> HHAADYVLYKDATKPVEDRVADLLGRMTLAEKIGQMTQIERLVATPDVLRDNFIGSLLSGGGSVPRKGATAKEWQDMVDGFQKACMSTRLGIPMIYGIDAVHGQNNVYGATIFPHNVGLGATRDPYLVKRIGEATALEVRATGIQYAFAPCIAVCRDPRWGRCYESYSEDRRIVQSMTELIPGLQGDVPKDFTSGMPFVAGKNKVAACAKHFVGDGGTVDGINENNTIINREGLMNIHMPAYKNAMDKGVSTVMISYSSWNGVKMHANQDLVTGYLKDTLKFKGFVISDWEGIDRITTPAGSDYSYSVKASILAGLDMIMVPNKYQQFISILTGHVNGGVIPMSRIDDAVTRILRVKFTMGLFENPYADPAMAEQLGKQEHRDLAREAARKSLVLLKNGKTSTDAPLLPLPKKAPKILV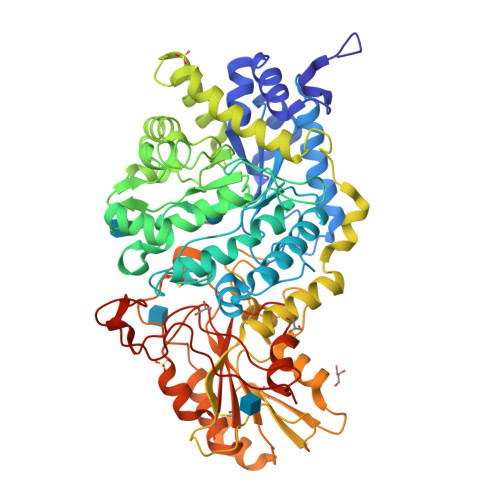AGSHADNLGYQCGGWTIEYQGDTGRTTVGTTILEAVKAAVDPSTVVVFAENPDAEFVKSGGFSYAIVAVGEHPYTETKGDNLNLTIPEPGLSTVQAVCGGVRCATVLISGRPVVVQPLLAASDALVAAWLPGSEGQGVTDALFGDFGFTGRLPRTWFKSVDQLPMNVGDAHYDPLFRLGYGLTTNATKKY>[2x]GAPIHDPDFIGGIGKELIVDNASDVTSFYPSAFQEHLNFIPAPTTGSGCTR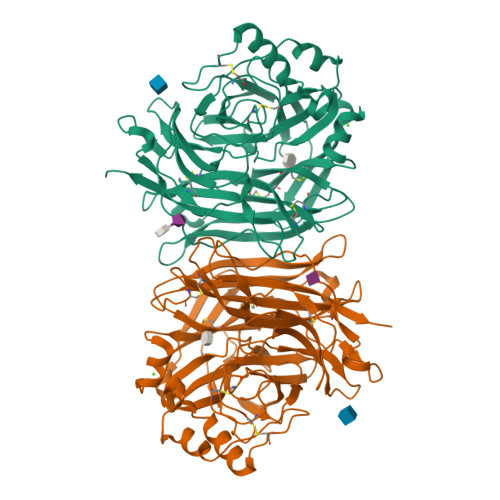IPSFDMSATHYCYTHNVILSGCRDHSHSHQYLALGVLRTTATGRIFFSTLRSISLDDTQNRKSCSVSATPLGCDMLCSKVTETEEEDYNSAVPTLMAHGRLGFDGQYHEKDLDVTTLFEDWVANYPGVGGGSFIDGRVWFSVYGGLKPNSPSDTVQEGKYVIYKRYNDTCPDEQDYQIRMAKSSYKPGRFGGKRIQQAILSIKVSTSLGEDPVLTVPPNTVTLMGAEGRILTVGTSHFLYQRGSSYFSPALLYPMTVSNKTATLHSPYTFNAFTRPGSIPCQASARCPNSCVTGVYTDPYPLIFYRNHTLRGVFGTMLDSEQARLNPASAVFDSTSRSRITRVSSSSTKAAYTTSTCFKVVKTNKTYCLSIAEISNTLFGEFRIVPLLVEILKNDGVREARSG>[2x]SNAMTEI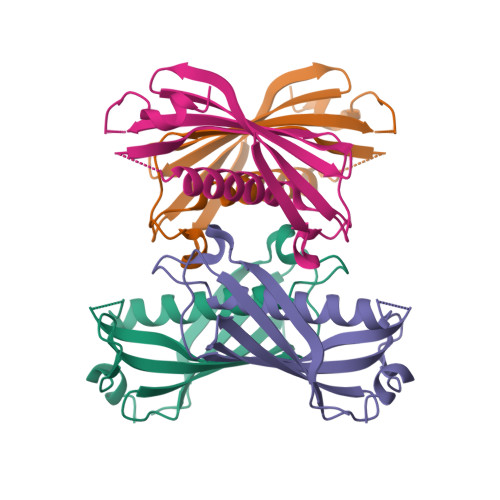NKIIHKKTFDIAWGDMAALGHVNNARYFDYFQEARIDWLRELDIKMTGQTGPVVIHVACTFLKPIVYPATVTIHSKVNSLGNSSMIMDHDLYQEETLMAQGVSKIVWIDYTQNKSVPLPDIIRNLV>[4x]ANPCCSNPCQNRGECMSTGFDQYKCDCTRTGFYGENCTTPEFLTRIKLLLKPTPNTVHYILTHFKGVWNIVNNIPFLRSLIMKYVLTSRSYLIDSPPTYNVHYGYKSWEAFSNLSYYTRALPPVADDCPTPMGVKGNKELPDSKEVLEKVLLRREFIPDPQGSNMMFAFFAQHFTHQFFKTDHKRGPGFTRGLGHGVDLNHIYGETLDRQHKLRLFKDGKLKYQVIGGEVYPPTVKDTQVEMIYPPHIPENLQFAVGQEVFGLVPGLMMYATIWLREHNRVCDILKQEHPEWGDEQLFQTSRLILIGETIKIVIEDYVQHLSGYHFKLKFDPELLFNQQFQYQNRIASEFNTLYHWHPLLPDTFNIEDQEYSFKQFLYNNSILLEHGLTQFVESFTRQIAGRVAGGRNVPIAVQAVAKASIDQSREMKYQSLNEYRKRFS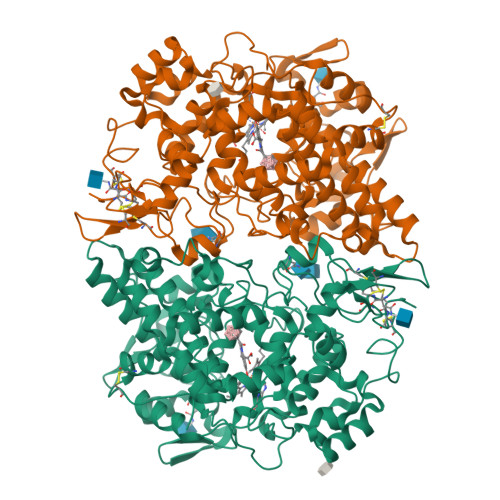LKPYTSFEELTGEKEMAAELKALYSDIDVMELYPALLVEKPRPDAIFGETMVELGAPFSLKGLMGNPICSPQYWKPSTFGGEVGFKIINTASIQSLICNNVKGCPFTSFNVQDPQPTKTATINASASHSRLDDINPTVLIKRRSTEL> HHHHHHSSGLVPRGSHMASDTIRIPGIDTPLSRVALGTWAIGGWMWGGPDDDNGVRTIHAALDEGINLIDTAPVYGFGHSEEIVGRALAEKPNKAHVATKLGLHWVGEDEKNMKVFRDSRPARIRKEVEDSLRRLRVETIDLEQIHWPDDKTPIDESARELQKLHQDGKIRALGVSNFSPEQMDIFREVAPLATIQPPLNLFERTIEKDILPYAEKHNAVVLA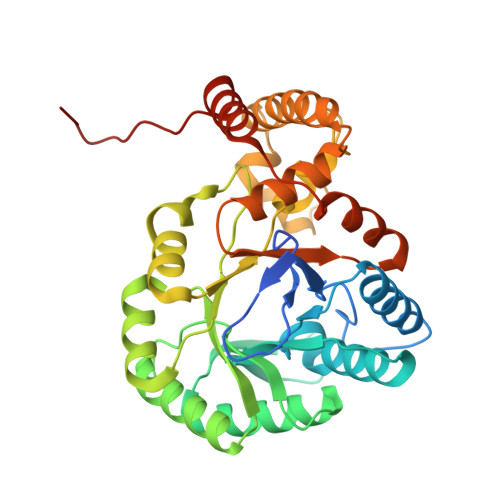YGALCRGLLTGKMNRDTTFPKDDLRSNDPKFQKPNFEKYLAAMDEFEKLAEKRGKSVMAFAVRWVLDQGPVIALWGARKPGQVSGVKDVFGWSLTDEEKKAVDDILARHVPNPIDPTFMAPPARD> VKSKAKKTVDKHSDEYKIRRER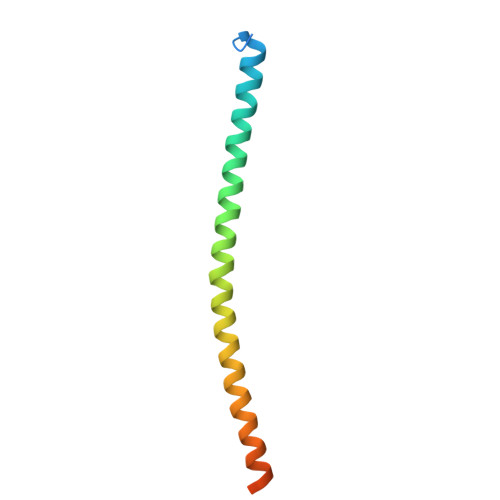NNIAVRKSRDKAKMRNLETQHKVLELTAENERLQKKVEQLSRELSTLRNLFKQLPEPLLASSGHC> MELFDENYYAKAVANIIGEVKDPIMYKWFSPDQIEDVDLQMGYQ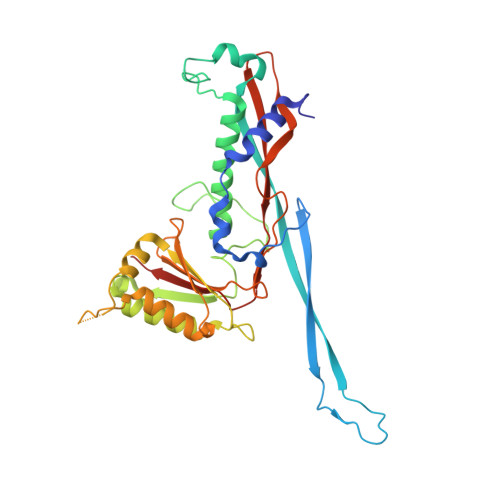KTVKWDAFLNANPTTIANEVNTISTIGFSSEVVRLNYLKLQYKFRHLKQTSEKFYTSDSYIGDINNNLLPFAQAYKLASSEIIKLINHFVLTGTVSIQKDGKNQKRLLPNMYGLLNMPEQIKEEVASGDKDKMDKIFEKIEAGLSKLELGDEFSTPMMVIVDPATSLKLVKPYAAAQGAASSCEKWEDVLIQTIKAINNREDVYIETSNLLKHKILIYPLNSELIKFKPSKYMLPTPNEQVDKDSTDVAHSYIDFVLGGLLATRKTILQVNIKQS> GPEIVDTCSLASPASVCRTKHLHLRCSVDFTRRTLTGTAALTVQSQEDNLRSLVLDTKDLTIEKVVINGQEVKYALGERQSYK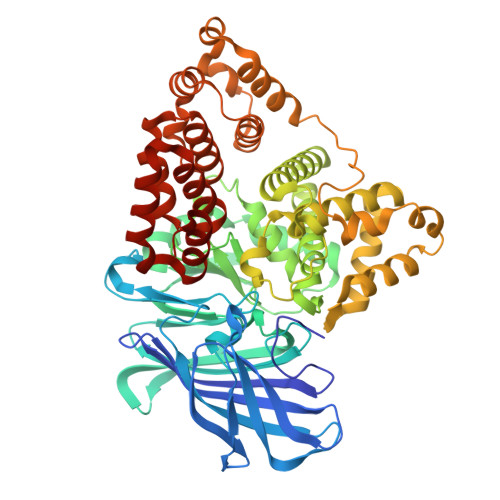GSPMEISLPIALSKNQEIVIEISFETSPKSSALQWLTPEQTSGKEHPYLFSQCQAIHCRAILPCQDTPSVKLTYTAEVSVPKELVALMSAIRDGETPDPEDPSRKIYKFIQKVPIPCYLIALVVGALESRQIGPRTLVWSEKEQVEKSAYEFSETESMLKIAEDLGGPYVWGQYDLLVLPPSFPYGGMENPCLTFVTPTLLAGDKSLSNVIAHQISHSWTGNLVTNKTWDHFWLNEGHTVYLERHICGRLFGEKFRHFNALGGWGELQNSVKTFGETHPFTKLVVDLTDIDPDVAYSSVPYEKGFALLFYLEQLLGGPEIFLGFLKAYVEKFSYKSITTDDWKDFLYSYFKDKVDVLNQVDWNAWLYSPGLPPIKPNYDMTLTNACIALSQRWITAKEDDLNSFNATDLKDLSSHQLNEFLAQTLQRAPLPLGHIKRMQEVYNFNAINNSEIRFRWLRLCIQSKWEDAIPLALKMATEQGRMKFTRPLFKDLAAFDKSHDQAVRTYQEHKASMHPVTAMLVGKDLKVD>MYSFEQAITQLFQQLSLSIPDTIEPVIGVKVGEFACHITEHPVGQILMFTLPSLDNNDEKETLLSHNIFSQDILKPILSWDEV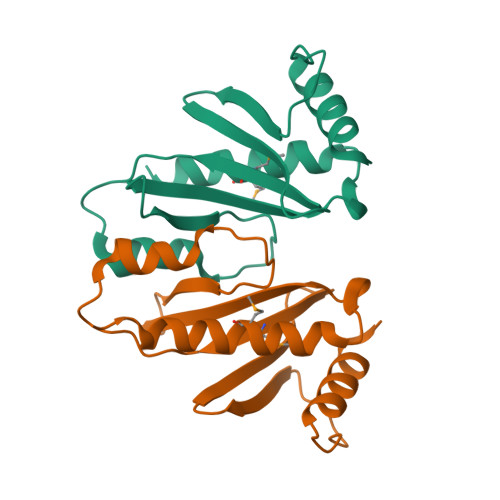GGHPVLWNRQPLNSLDNNSLYTQLEMLVQGAERLQTSSLISPPRSFS[2x]>ALYEDPPDQKTSPSGKPATLKICSWNVDGLRAWIKKKGLDWVKEEAPDILCLQETKCSENKLPAELQELPGLSHQYWSAPSDKEGYSGVGLLSRQCPLKVSYGIGDEEHDQEGRVIVAEFDSFVLVTAYVPNAGRGLVRLEYRQRWDEAFRKFLKGLASRKPLVLCGDLNVAHEEIDLRNPKGNKKNAGFTPQERQGFGELLQAVPLADSFRHLYPNTPYAYTFWTYMMNARSKNVGWRLDYFLLSHSLLPALCDSKIRSKAL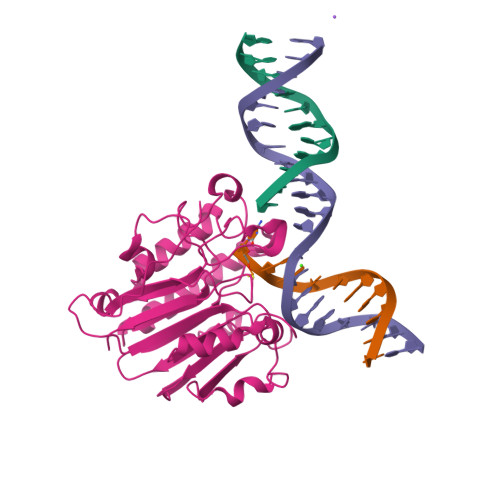GSDHCPITLYLAL[2x]> ENQYV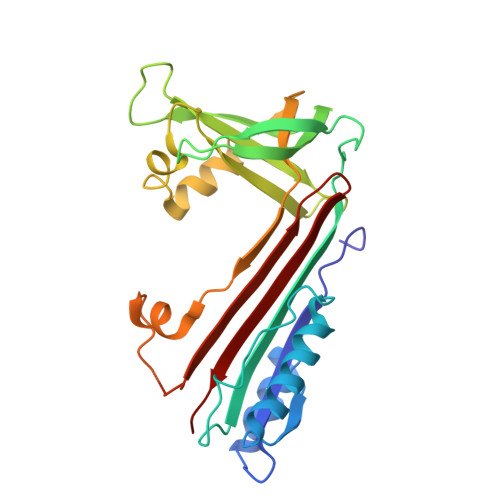MKLANSLFVQNGFHVNEEFLQMLKMYFNAEVNHVDFSQNVAVANSINKWVENYTNSLLKDLVSPEDFDGVTNLALINAVYFKGNWKSQFRPENTRTFSFTKDDESEVQIPMMYQQGEFYYGEFSDGSNEAGGIYQVLEIPYEGDEISMMLALSRQEVPLATLEPLLKAQLIEEWANSVKKQKVEVYLPRFTVEQEIDLKDILKALGVTEIFIKDANLTAMSDKKELFLSKAVHKSCIEVNEEGSEAAAASGMIAIS>[3x]MSPIPNRVSSGSLADAVFKSACEERILLAYADYNPDMTKVVNLFSKYNETVNTVRVSNDAVKDILEIVGWPSMPLIFVKGNCCGGFKELYQLEESGFLNEWLKEHEYDLAIVGGGSGGLAAAKEAVRLGKKVVCLDFVKPSAMGTTWGL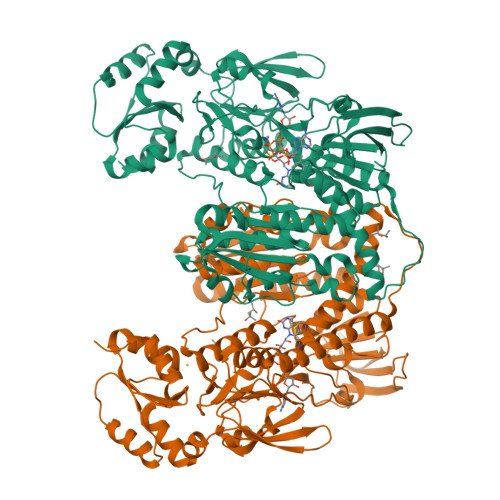GGTCVNVGCIPKKLMHQAALLGEYIEDAKKFGWEIPEGAIKLNWHQLKNAVQNHIASLNWGYRVQLKEKSVTYMNSYATFTGSHELSVKNKKGKVEKVTADRFLIAVGLRPRFPDVPGALECCISSDDLFSLPYNPGKTLCVGASYVSLECAGFLKGIGNDVTVMVRSVLLRGFDQDMAERIKKHMTERGVKFVQCVPIKYERLKKPTDSEPGMIRVHTMQEDEDGTKEVTEDFNTVLMAIGRDAMTDDLGLDVVGVNRAKSGKIIGRREQSVSCPYVYAIGDVLYGSPELTPVAIQAGKVLMRRLFTGSSELTEYDKIPTTVFTPLEYGSCGLSEYSAIQKYGKENINVYHNVFIPLEYAVTERKEKTHCYCKLICLKNEQDLILGFHILTPNAGEITQGFAIALKFDAKKADFDRLIGIHPTVAENFTTLTLVKEDGQTLKATGCUG> MGLCLAKRNHDADDDEPHIELAGGNVHLITTKERWDQKLSEASRDGKIVLANFSARWCGPSRQIAPYY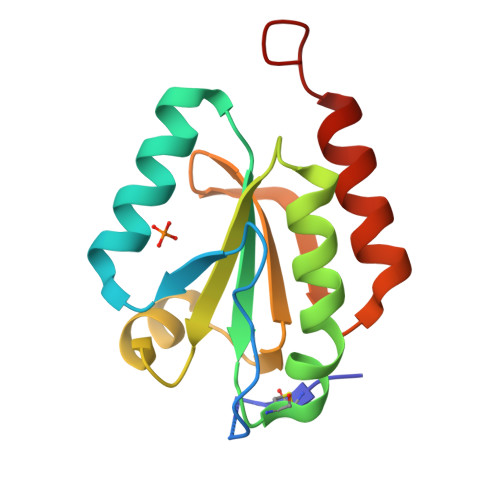IELSENYPSLMFLVIDVDELSDFSASWEIKATPTFFFLRDGQQVDKLVGANKPELHKKITAILDSLPPSDK> AIEKRLASLLTGQGLAFRVQDASLPGRPDFVVDEYRCVIFTHGCFWHHHHCY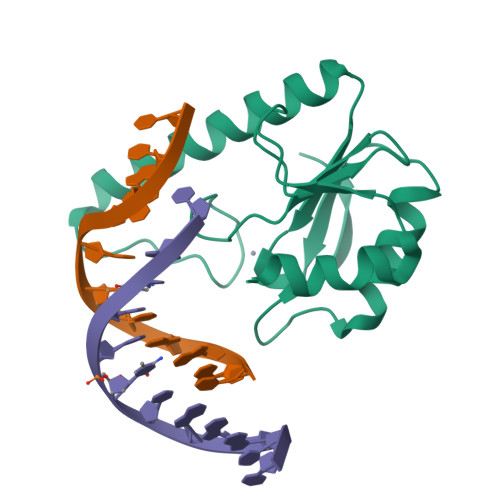LFKVPATRTEFWLEKIGKNVERDRRDISRLQELGWRVLIVWECALRGREKLTDEALTERLEEWICGEGASAQIDTQGIHLLA>GMSEPEVPFKVVAQFPYKSDYEDDLNFEKDQEIIVTSVEDAEWYFGEYQDSNGDVIEGIFPKSFVAVQG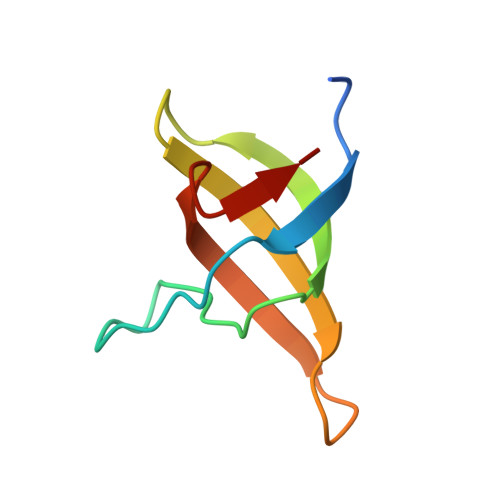[4x]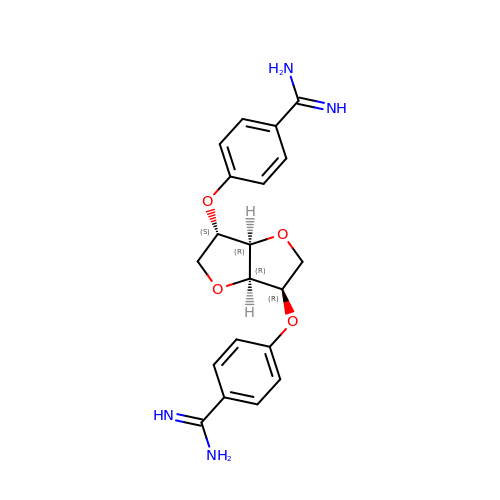2,5-BIS-O-{4-[AMINO(IMINO)METHYL]PHENYL}-1,4:3,6-DIANHYDRO-D-GLUCITOL | C20 H22 N4 O4 | CDEVHSIVANGYRI-XMTFNYHQSA-N> GGCGUGGUCCG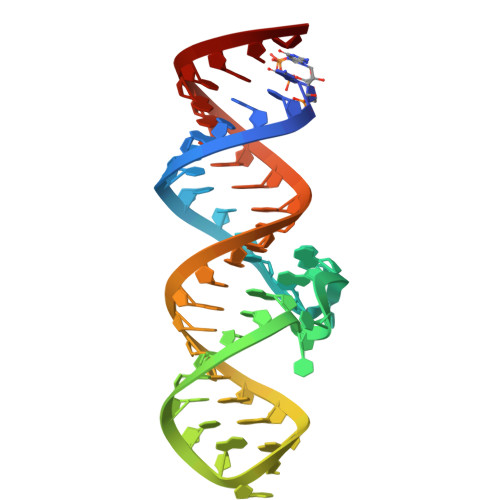UUCAAGUCGUUCCUCGAAAGAGGAACUACGGGAGACGCC~{N}-oxidanyl-4-phenanthridin-6-yl-benzamide | 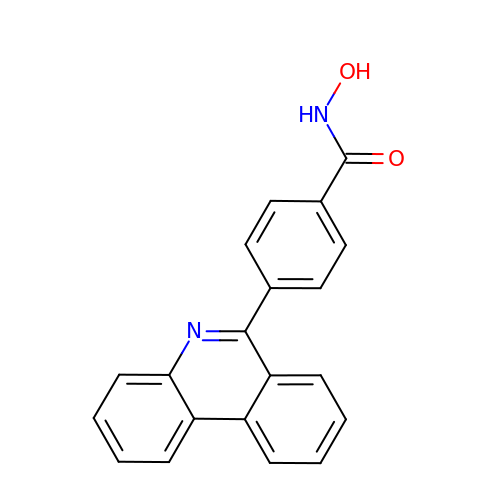C20 H14 N2 O2 | SKTQGZRQWBQSQM-UHFFFAOYSA-N(2E,4E,6E,8E)-9-(4-hydroxy-2,3,6-trimethylphenyl)-3,7-dimethylnona-2,4,6,8-tetraenoic 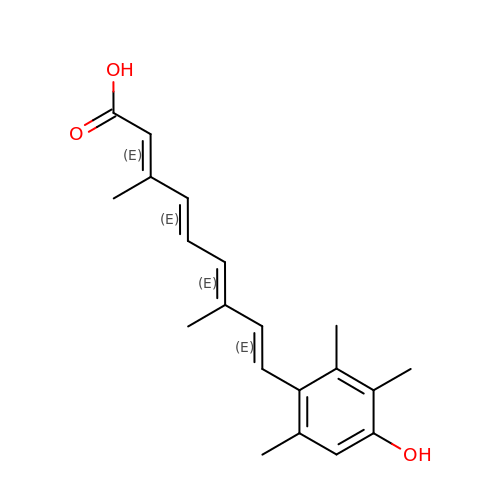acid | C20 H24 O3 | CAAFTBWHFUPDGX-OFCLTBKTSA-N>[3x]SGPRPRLWEGQDVLARWTDGLLYLGTIKKVDSAREVCLVQFEDDSQFLVLWKDISPAALPGEELLCCVCRSETVVPGNRLVSCEKCRHAYHQDCHVPRAPAPGEGEGTSWVCRQCVFAIATKRGGALKKGPYARAMLGM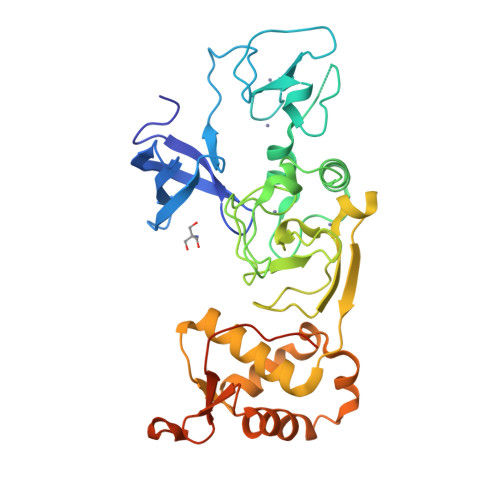KLSLPYGLKGLDWDAGHLSNRQQSYCYCGGPGEWNLKMLQCRSCLQWFHEACTQCLSKPLLYGDRFYEFECCVCRGGPEKVRRLQLRWVDVAHLVLYHLSVCCKKKYFDFDREILPFTSENWDSLLLGELSDTPKGERSSRLLSALNSHKDRFISGREIKKRKCLFGLHARMPPPVEPPTGDGALTSFPSGQGPGGG>HHHHHHMPIPVGNTKNDFAALQA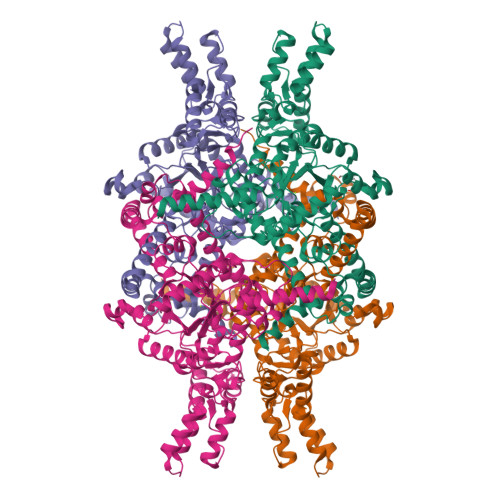KLDADAAEIEKWWSDSRWSKTKRNYSARDIAVRRGTFPPIEYPSSVMARKLFKVLEKHHNEGTVSKTFGALDPVQISQMAKYLDTIYISGWQCSSTASTSNEPGPDLADYPMDTVPNKVEHLFKAQLFHDRKQLEARSKAKSQEELDEMGAPIDYLTPIVADADAGHGGLTAVFKLTKMFIERGAAGIHMEDQTSTNKKCGHMAGRCVIPVQEHVNRLVTIRMCADIMHSDLIVVARTDSEAATLISSTIDTRDHYFIVGATNPNIEPFAEVLNDAIMSGASGQELADIEQKWCRDAGLKLFHEAVIDEIERSALSNKQELIKKFTSKVGPLTETSHREAKKLAKEILGHEIFFDWELPRVREGLYRYRGGTQCSIMRARAFAPYADLVWMESNYPDFQQAKEFAEGVKEKFPDQWLAYNLSPSFNWPKAMSVDEQHTFIQRLGDLGYIWQFITLAGLHTNALAVHNFSRDFAKDGMKAYAQNVQQREMDDGVDVLKHQKWSGAEYIDGLLKLAQGGVSATAAMGTGVTEDQFKENGVKK[4x]>[4x]MNLLSDKNVAIIGGGPVGLTMAKLLQQNGIDVSVYERDNDREARIFGGTLDLHKGSGQEAMKKAGLLQTYYDLALPMGVNIADKKGNILSTKNVKPENRFDNPEINRNDLR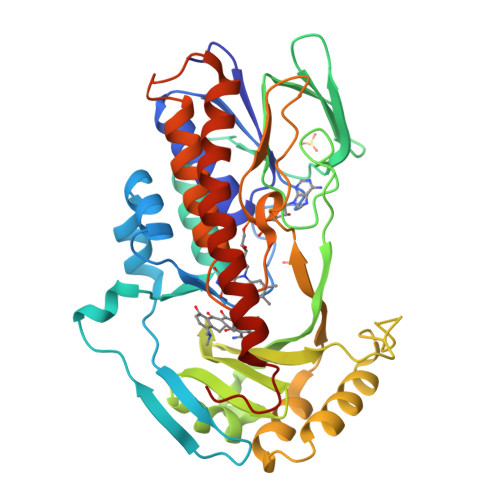AILLNSLENDTVIWDRKLVMLEPGKKKWTLTFENKPSETADLVILANGGMSKVRKFVTDTEVEETGTFNIQADIHQPEINCPGFFQLCNGNRLMASHQGNLLFANPNNNGALHFGISFKTPDEWKNQTQVDFQNRNSVVDFLLKKFSDWDERYKELIHATLSFVGLATRIFPLEKPWKSKRPLPITMIGDAAHLMPPFAGQGVNSGLVDALILSDNLADGKFNSIEEAVKNYEQQMFIYGKEAQEESTQNEIEMFKPDFTFQQLLNV> SNAMNDIILKSLSTLITEQRNPNSVDIDRQSTLEIVRLMNEEDKLVPLAIESCLPQISLAVEQIVQAFQQGGRLIYIGAGTSGRLGVLDASECP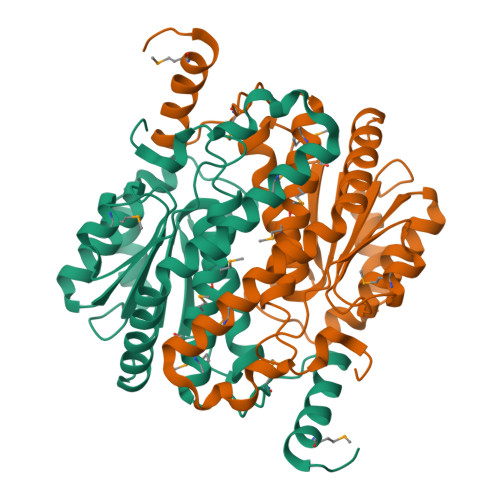PTFGVSTEMVKGIIAGGECAIRHPVEGAEDNTKAVLNDLQSIHFSKNDVLVGIAASGRTPYVIAGLQYAKSLGALTISIASNPKSEMAEIADIAIETIVGPEILTGSSRLKSGTAQKMVLNMLTTASMILLGKCYENLMVDVQASNEKLKARAVRIVMQATDCNKTLAEQTLLEADQNAKLAIMMILSTLSKSEAKVLLERHQGKLRNALSK>MGSSHHHHSQASMITRYKPESGFVARSGGPDRKRPHDWIVWHFTHADNLPGIITAGRLLADSAVTPTTEVAYNPVKELRRHKVVAPDSRYPASMASDHVPFYIAARSPMLYVVCKGHSGYSGGAGPLVHLGVALGDIIDADLTWCASDGNAAASYTKFSRQVDTLGTFVDFDLLCQRQWHNTDDDPNRQSRRAAAILVYGHVPFELVSYVCCYNTETMTRVRTLLDPVGGVRKYVIKPGMYY[2x];>MTWGRAVILEAMRRYLQQRRAMEPWEDPAGISHLEIQKLMY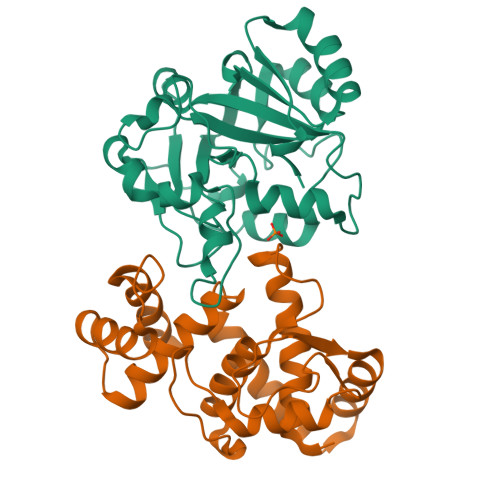FANEADPDLALDFTPGRYGPYSERVRHLLQGMEGAFTVGLGDGTARVLANQPISLTTKGTDAITDYLATDAAADRVSAAVDTVLRVIEGFEGPYGVELLASTHWVATREGAKEPATAAAAVRKWTKRKGRIYSDDRIGVALDRILMTA[2x]The essential membrane protein complex of FtsB, FtsL and FtsQ (FtsBLQ) is at the heart of the divisome assembly cascade in Escherichia coli. This complex regulates the transglycosylation and transpeptidation activities of the FtsW-FtsI complex and PBP1b via coordination with FtsN, the trigger for the onset of constriction. A core complex at the heart of this machinery is composed of three type-II bitopic membrane proteins, the Filamentous temperature-sensitive proteins B, L and Q (FtsB, FtsL, FtsQ). For a long time, the FtsBLQ complex was believed to act as a non-enzymatic scaffold for the assembly of the divisome, but recent studies revealed it to be a positive regulator of the FtsWI complex and a negative regulator of the bi-functional PG synthase PBP1b.

The crystal structure of the FtsBLQ complex was determined at 3.1 Å resolution by molecular replacement using the partial structure of the complex as the input model, which contains the periplasmic domain of FtsQ and the C-terminal region of FtsB (PDB: 5Z2W18). The remaining atoms (~40%) were manually built, including three fully resolved transmembrane (TM) helices. The three proteins of the complex, in a stoichiometry of 1:1:1, meet at the C-terminal membrane-distal region and form an inverted V-shape conformation. One branch of the V-shape is a lengthy coiled-coil heterodimer FtsB-FtsL (FtsBL), which extends continuously from the inner membrane to the periplasmic, where their key functional domains locate. The other branch comes from FtsQ that adopts a rod-like shape, with two globular periplasmic domains arranged linearly and connected to the TM helix α1 in a slightly bent manner. The crossing point of the two branches, however, is not at the very tip but somewhere in the middle of the continuous FtsBL coiled coil, forming an included angle of ~37°, where an interface between FtsB and FtsQ is revealed. Therefore, the two rigid periplasmic branches of FtsBLQ form an obtuse triangle with the plane of the membrane (49 Å and 70 Å in length and at ~37° angle) and are connected to the bendable FtsQ-TM and the unbendable FtsBL-TM on each side. In Site I, a heterotrimeric β-sheet is revealed for the first time in the FtsBLQ complex, involving three C-terminal β-strands, FtsLE115–V118, FtsBE83–P88, FtsQS250–W256. The tightly bent short helix of FtsB-α3 is sandwiched by the short helix of FtsL-α2 and the β domain of FtsQ, forming an extensive hydrogen-bond/electrostatic interaction network which involves the FtsB-FtsQ interface near the C-terminus of the coiled coil. Therein, FtsBE56 serves as an interaction hot spot, bringing together the β8-β9 and β10-α6 linkers of FtsQ, the α3 helix of FtsB, the α2 helix of FtsL, and the C-terminal region of the coiled coil.

> MGSSHHHHHHSQDPNSMGKLTLLLLAILVWLQYSLWFGKNGIHDYTRVNDDVAAQQATNAKLKARNDQLFAEIDDLNGGQEALEERARNELSMTRPGETFYRLVPDASKRAQSAGQNNR;> MISRVTEALSKVKGSMGSHERHALPGVIGDDLLRFGKLPLCLFICIILTAVTVVTTAHHTRLLTAQREQLVLERDALDIEWRNLILEENALGDHSRVERIATEKLQMQHVDPSQENIVVQK;> MSQAALNTRNSEEEVSSRRNNGTRLAGILFLLTVLTTVLVSGWVVLGWMEDAQRLPLSKLVLTGERHYTRNDDIRQSILALGEPGTFMTQDVNIIQTQIEQRLPWIKQVSVRKQWPDELKIHLVEYVPIARWNDQHMVDAEGNTFSVPPERTSKQVLPMLYGPEGSANEVLQGYREMGQMLAKDRFTLKEAAMTARRSWQLTLNNDIKLNLGRGDTMKRLARFVELYPVLQQQAQTDGKRISYVDLRYDSGAAVGWAPLPPEESTQQQNQAQAEQQ>[2x]HHHHHHSSGMVFYFTSSSVNSSAYT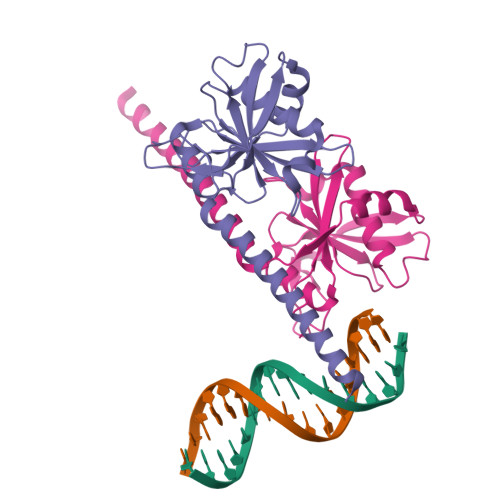IYMGKDKYENEDLIKHGWPEDIWFHVDKLSSAHVYLRLHKGENIEDIPKEVLMDCAHLVKANSIQGCKMNNVNVVYTPWSNLKKTADMDVGQIGFHRQKDVKIVTVEKKVNEILNRLEKTKVERFPDLAAEKECRDREERNEKKAQIQEMKKREKEEMKKKREMDELRS> MDILRKVAEIHGTPTYVYFEETLRKRSRLVKEVFEGVNLLPTFAVKANNNPVLLKILREEGFGMDVVTKGELLAAKLAGVPSHTVVWNGNGKSRDQMEHFLREDVRIVNVDSFEEMEIWRELNPEGVEYFIRVNPEVDAKTHPHISTGLKKHKFGIPLEDLDSFMERFRSMNIRGLHVHIGSQITRVEPFVE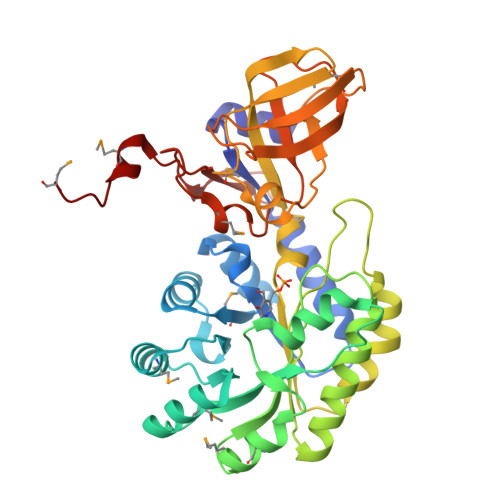AFSKVVRASERYGFEEINIGGGWGINYSGEELDLSSYREKVVPDLKRFKRVIVEIGRYIVAPSGYLLLRVVLVKRRHNKAFVVVDGGMNVLIRPALYSAYHRIFVLGKQGKEMRADVVGPLCESGDVIAYDRELPEVEPGDIIAVENAGAYGYTMSNNYNSTTRPAEVLVRENGRISLIRRRETEMDIFKDVVM> GPLGSMMFLPTDYCCRLSDQEYMELVFENGQILAKGQR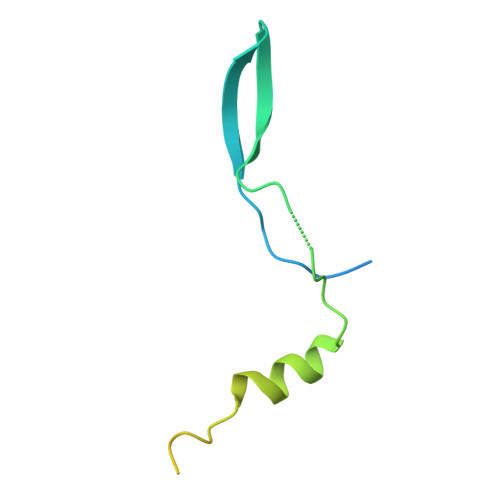SNVSLHNQRTKSIMDLYEAEYNEDFMKSIIHGGGGAITNLGDTQVVPQSHVAAAHETNMLESNKHVD>[4x]EQVFHFYWLDAYEDQYNQPGVVFLFGKVWIESAETHVSCCVMVKNIERTLYFLPREMKIDLNTGKETGTPISMKDVYEEFDEKIATKYKIMKFKSKPVEKNYAFEIPDVPEKSEYLEVKYSAEMPQLPQDLKGETFSHVFGTNTSSLELFLMNRKIKGPCWLEVKSPQLLNQPVSWCKVEAMALKPDLVNVIKDVSPPPLVVMAFSMKTMQNAKNHQNEIIAMAALVHHSFALDKAAPKPPFQSHFCVVSKPKDCIFPYAFKEVIEKKNVKVEVAATERTLLGFFLAKVHKIDPDIIVGHNIYGFELEVLLQRINVCKAPHWSKIGRLKRSNMPKLGGRSGFGERNATCGRMICDVEISAKELIRCKSYHLSELVQQILKTERVVIPMENIQNMYSESSQLLYLLEHTWKDAKFILQIMCELNVLPLALQITNIAGNIMSRTLMGGRSERNEFLLLHAFYENNYIVPDKQIFRKPQQKLGDEDEEIDGDTNKYKKGRKKAAYAGGLVLDPKVGFYDKFILLLDFNSLYPSIIQEFNICFTTVQRVASEAQKVTEDGEQEQIPELPDPSLEMGILPREIRKLVERRKQVKQLMKQQDLNPDLILQYDIRQKALKLTANSMYGCLGFSYSRFYAKPLAALVTYKGREILMHTKEMVQKMNLEVIYGDTDSIMINTNSTNLEEVFKLGNKVKSEVNKLYKLLEIDIDGVFKSLLLLKKKKYAALVVEPTSDGNYVTKQELKGLDIVRRDWCDLAKDTGNFVIGQILSDQSRDTIVENIQKRLIEIGENVLNGSVPVSQFEINKALTKDPQDYPDKKSLPHVHVALWINSQGGRKVKAGDTVSYVICQDGSNLTASQRAYAPEQLQKQDNLTIDTQYYLAQQIHPVVARICEPIDGIDAVLIATWLGLDPTQFRVHHYHKDE

Polα/primase is a four-subunit enzyme (p180, p70, p49 and p58 in humans) whose activity is absolutely required for cell viability. This complex assembles short RNA-DNA primers which are subsequently extended by the processive Polδ and Polε. As such, the Polα catalytic subunit encounters two types of DNA substrates during the primer synthesis: an RNA:DNA helix that is handed over to it by the primase subunits and then a DNA:DNA helix during subsequent DNA synthesis. Crystal structures of the catalytic subunits of Polα, Polδ, and Polε reveal a characteristic B-family polymerase fold comprised of a palm domain that carries the catalytic residues for dNTP addition, a fingers domain that drapes over the nascent base pair, a thumb domain that makes contacts in the DNA minor groove, and an N-terminal domain (NTD).

The catalytic core of hPolα (residues 339 to 1259 of the p180 subunit) was crystallized with a 13-nt primer DNA/18-nt template DNA from a mix containing Mg2+ and dCTP. There are four polymerase-DNA (binary) complexes in the crystallographic asymmetric unit. Unlike the ternary (polymerase-RNA/DNA-incoming nucleotide) structures where the fingers domain is draped over the nascent base-pair, the fingers domain in our structure is in the open conformation. When compared to the human Polα ternary structure, the fingers domain in our binary structure is rotated outwards by ~22°. Intriguingly, the templating guanine base is rotated about its glycosidic bond to the syn conformation. It is stabilized in this conformation by stacking interactions with the side chain of Arg784 from the NTD. Strikingly, the portion of DNA:DNA helix in contact with the polymerase has a mixed A-B conformation while the portion of the duplex outside of the contact region remains in the standard B-form. By contrast, the portion of the DNA:DNA helix outside the contact region remains in standard B-form. This suggests a model where Polα imposes a hybrid A-B-like conformation on the DNA:DNA helix rather than any major rearrangement in the polymerase to fit a B-form DNA. Almost all of the contacts noted previously with an RNA primer are preserved with a DNA primer9. The Polα catalytic core binds the two substrates with similar affinities, namely with a Kd of ~320 nM to the RNA:DNA helix and with a Kd of ~430 nM to the DNA:DNA helix.>MMFGRFTERAQKVLALAQEEALRLGHNNIGTEHILLGLVREGEGIAAKALQALGLGSEKIQKEVESLIGRGQEMSQTIHYTPRAKKVIELSMDEARKLGHSYVGTEHILLGLIREGEGVAARVLNNLGVSLNKARQQVLQLLGSNETGSSAAGTNSNANTPTLDSLARDLTAIAKEDSLDPVIGRSKEIQRVIEVLSRRTKNNPVLIGEPGVGKTAIAEGLAQQIINNEVPEILRDKRVMTLDMGTVVAGTKYRGEFEDRLKKVMDEIRQAGNIILFIDALHTLIGAGGAEGAIDASNILKPSLARGELQCIGATTLDEYRKYIEKDAALERRFQPIQVDQPSVDESIQILQGLRDRYEAHHRVSITDDAIEAAVKLSDRYISDRFLPDKAIDLIDEAGSKVRLRSFTTPPNLKELEQKLDEVRKEKDAAVQSQEFEKAASLRDTEQRLREQVEDTKKSWKEKQGQENSEVTVDDIAMVVSSWTGVPVSKIAQTETDKLLNMENILHSRVIGQDEAVVAVAKAVRRARAGLKDPKRPIGSFIFLGPTGVGKTELARALAESIFGDEESMIRIDMSEYMEKHSTSRLVGSPPGYVGYDEGGQLTEKVRRKPYSVVLLDA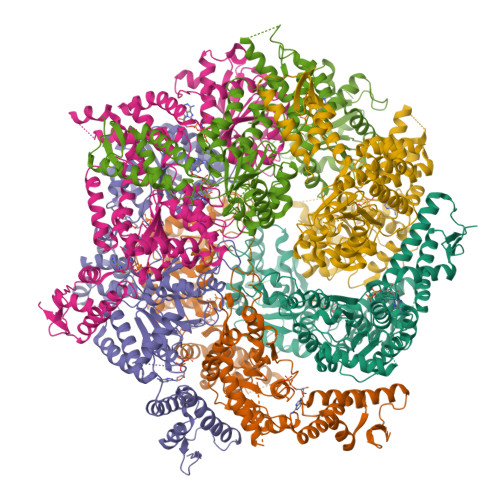IEKAHPDVFNILLQVLEDGRLTDSKGRTVDFRNTILIMTSNVGASELKRNKYVGFNVQDETQNHKDMKDKVMGELKRAFRPEFINRIDEIIVFHSLEKKHLTEIVSLMSDQLTKRLKEQDLSIELTDAAKAKVAEEGVDLEYGARPLRRAIQKHVEDRLSEELLRGNIHKGQHIVLDVEDGEFVVKTTAKTNLEHHHHHH[6x]4-(propanoylamino)-~{N}-[4-[(5,8,11-trimethyl-6-oxidanylidene-pyrimido[4,5-b][1,4]benzodiazepin-2-yl)amino]phenyl]benzamide | C30 H29 N7 O3 | 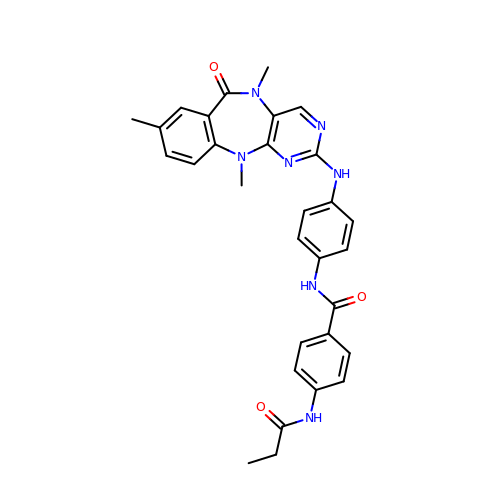KGXBCWANASZZQG-UHFFFAOYSA-N> VTKPTIAAVGGYAMNNGTGTTLYTKAADTRRSTGSTTKIMTAKVVLAQSNLNLDAKVTIQKAYSDYVVANNASQAHLI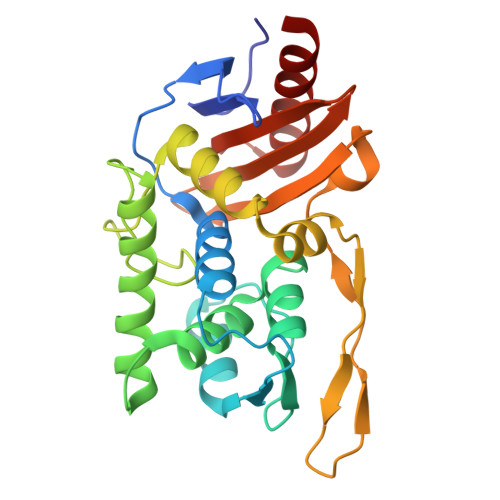VGDKVTVRQLLYGLMLPSGCDAAYALADKYGSGSTRAARVKSFIGKMNTAATNLGLHNTHFDSFDGIGNGANYSTPRDLTKIASSAMKNSTFRTVVKTKAYTAKTVTKTGSIRTMDTWKNTNGLLSSYSGAIGVKTGAGPEAKYCLVFAATRGGKTVIGTVLASTSIPARESDATKIMNYGFAL3,5-dichloro-4-hydroxybenzene-1-sulfonic acid | C6 H4 Cl2 O4 S | 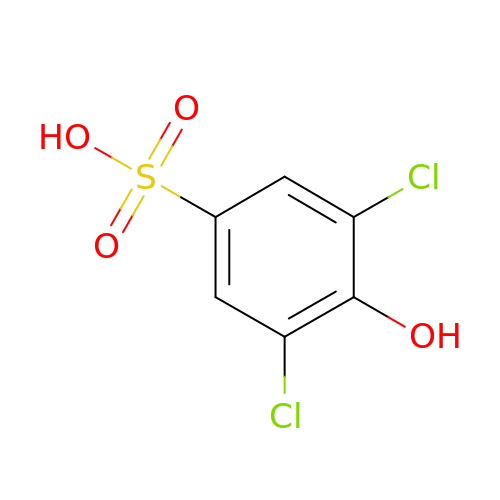PGDCAFRJYQICAY-UHFFFAOYSA-N> XWKRHIS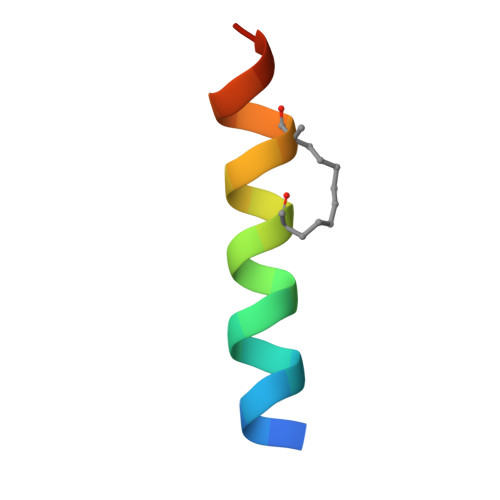EQLRLRDRLQRQAFEX>[6x]MKSEKEKMLAGHLYNPADLELVKERERARRLVRLYNETLETEYDKRTGLLKELFGSTGERLFIEPNFRCDYGYNIHVGENFFMNFDGVILDVCEVRIGDHCFIGPGV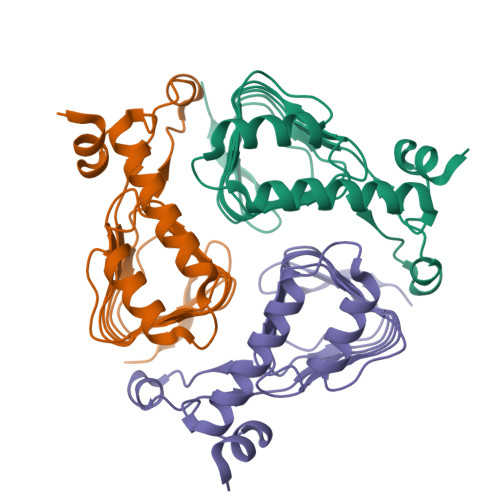HIYTATHPLDPHERNSGLEYGKPVVIGHNVWIGGRAVINPGVTIGDNAVIASGAVVTKDVPANAVVGGNPAKVIKWLK> NNKRAPYWTNTEKMEKRLHAVPAANTVKFRCPAGGNPMPT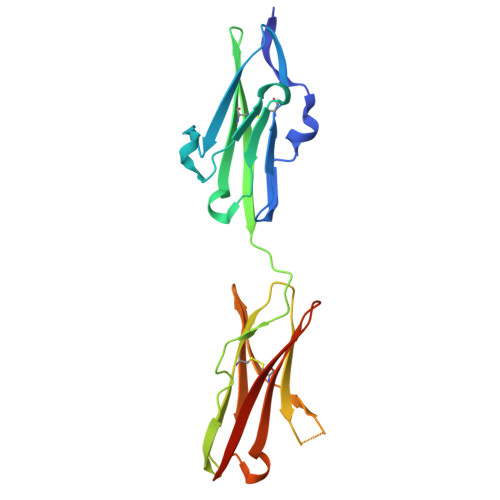MRWLKNGKEFKQEHRIGGYKVRNQHWSLIMESVVPSDKGNYTCVVENEYGSINHTYHLDVVERSRHRPILQAGLPANASTVVGGDVEFVCKVYSDAQPHIQWIKHVEKNGSKYGPDGLPYLKVLKAAGVNTTDKEIEVLYIRNVTFEDAGEYTCLAGNSIGISFHSAWLTVLPAPGREKE> DPAMQRCFSAAVYCA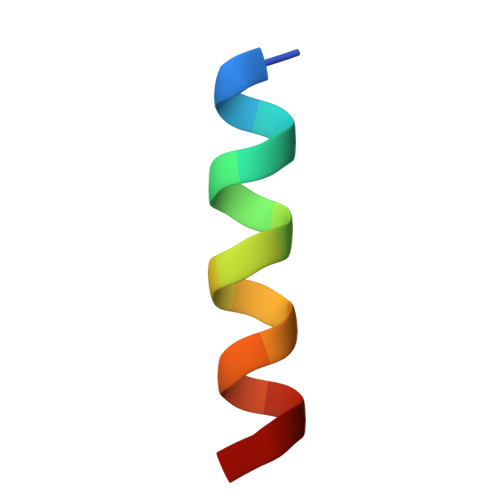IS> TQVHMLYINAEVNGISIKAFVDSGAQTTIMSKKCAEKCNLVRLIDYRFSGIAQGVGTSKIVGKIHVAQMKIGNSFFPFSITVLEESHVDFLFGLDLLKRYQCCIDLHQNALIIGDE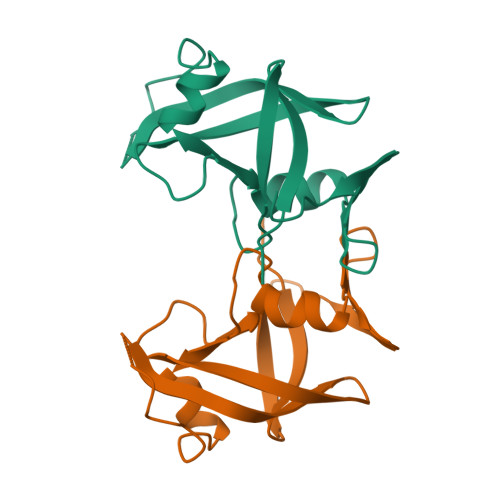KVQFLSESEINS> XMDSE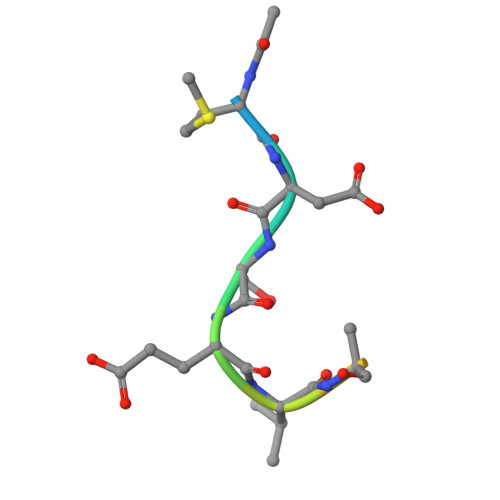VAALVID>[2x]MGNERLDELRARVDEINLQLLKLINERGRLVQEIGKIKEAQG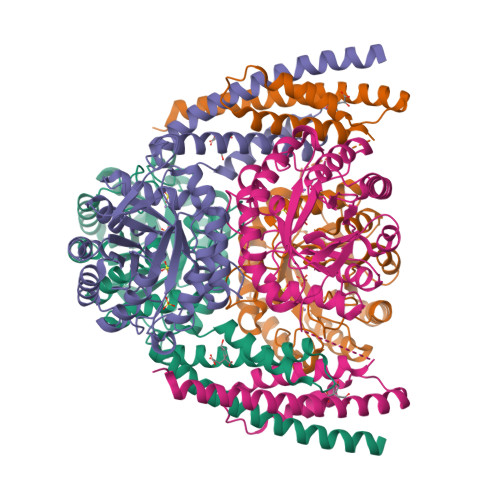THRYDPVRERKMLDLISEHNDGPFETSTLQHIFKEIFKAALELQEDDHRKALLVSRKKHPENTIVEVKGERIGDGNQYFVMGPCAVESYEQVAAVAEAVKKQGIKLLRGGAYKPRTSPYDFQGLGVEGLKILKRIADEFDLAVISEIVTPADIEIALDYIDVIQIGARNMQNFELLKAAGQVNKPILLKRGLAATIEEFINAAEYIMSQGNGQIILCERGIRTYERATRNTLDISAVPILKKETHLPVFVDVTHSTGRRDLLIPCAKAALAIGADGVMAEVHPDPAVALSDSAQQMDIAQFNEFMEEVRAFQRQFVRALEHHHHHH> GRSDAYTQVDNFLHAYARGGDELVNGHPSYTVDQAAEQILREQASWQKAPGDSVLTLSYSFLTKPNDFFNTPWKYVSDIYSLGKFSAFSAQQQAQAKLSLQSWSDVTNIHFVDAGQGDQGDLTFGNFSSSVGGAAFAFLPDVPDALKGQSWYLINSSYSANVNPANGNYGRQTLTHEIGHTLGLSHPGDYNAGEGDPTYADATYAEDTRAYSVMSYWEEQNTGQDFKGAYSSAPLLDDIAAIQKLYGANLTTRTGDTVYGFNSNTERDFYSATSSSSKLVFSVWDAGGNDTLDFSGFSQNQKINLNEKALSDVGGLKGNVSIAAGVTVENAIGGSGSDLLIGNDVANVLKGGAGNDILYGGLGADQLWGGAGADTFVYGDIAESSAAAPDTLRDFVSGQDKIDLSGLDAFVNGGLVLQYVDAFAGKAGQAILSY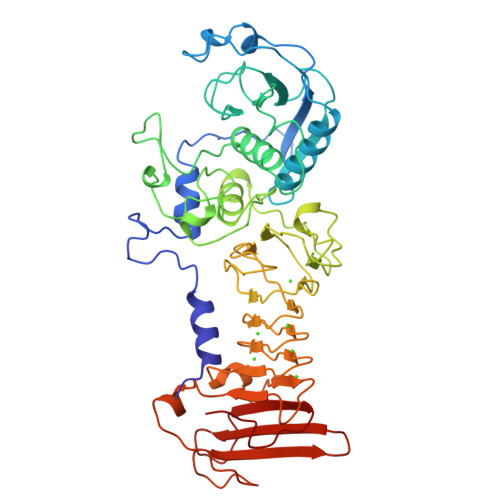DAASKAGSLAIDFSGDAHADFAINLIGQATQADIVV> GIDPFTMADDLPPAPVITAQASVPLTSESFVAAAVSRSGPAVVRIDTETVVTRRTDPILDDPFFQEFFGRSFPVPPRERRIAGQGSGFIIDNSGIILTNAHVVDGASKVVVTLRDGRTFDGQVRGTDEVTDLAVVKIEPQGSALPVAPLGTSSNLQVGDWAIAVGNPVGLDNTVTLGIISTLGRSAAQAGIPDKRVEFIQTDAAINPGNSGGPLLNAR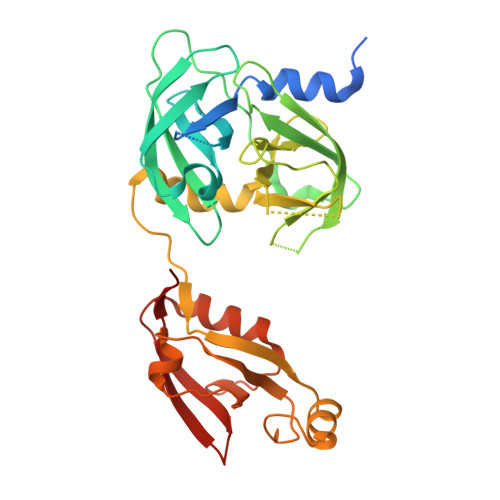GEVIGINTAIRADATGIGFAIPIDQAKAIQNTLAAGGTVPHPYIGVQMMNITVDQAQQNNRNPNSPFIIPEVDGILVMRVLPGTPAERAGIRRGDVIVAVDGTPISDGARLQRIVEQAGLNKALKLDLLRGDRRLSLTVQTAQLRNPTS>MSSVSIFGLGAMGTALASRFLEEKYKVAVWNRSPEKASSLLGKGATLSHTAVDGINASDLIIICLLDNAAVEATLAGALDHLHGKTIINLTNGTPDQARKLSDRFVSHGARYVHGGIMATPSMIGSPYALVLYSGSPDAFKAAEGDLSVLAKCVFLGEDAGTASLHDLALLSGMYGLFSGFLHATALVRSSTPAVKFMDLLVPWLGAMTEYTKGMAKQIDEGKYTSEGSNLAMQLVGIQNIIDASEAQQVSAEFIRPMKEFMQKAVAAGHGG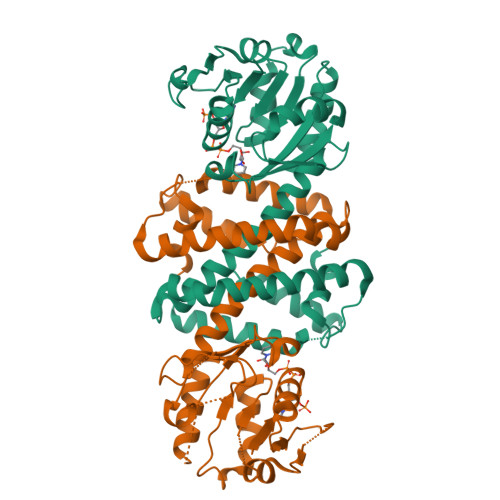DDISSLIDFVKST[8x]> GKLYLNHSAKQHTSASDHLLTEISVNHGEHKQVTLPDGTVVHLNAGTVMRYPTEFTSDIRL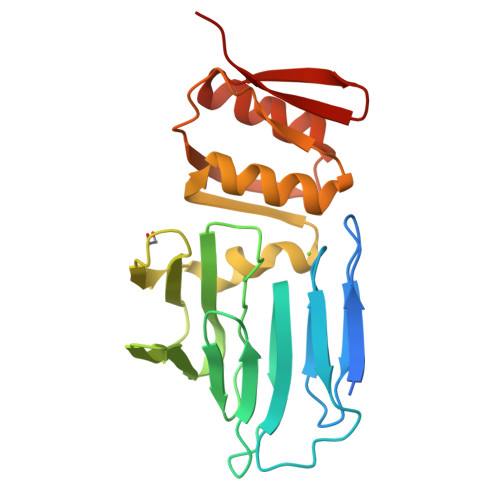VEMEGEAFFNVMRDEGKPFIVRTRQADVKVLGASFNVKAYQEDELMAVSVRTGKVEVDMPESVMRLLPNEQIIVNNTNGEILKKNEDAQKVTAWLQGGLYFNRTPISSVIHDLERMYNQEIVLDPNVVFDDYIYGEHDNKSLEAVLNAIQYSTGIRYRKEESRIVLYKTSH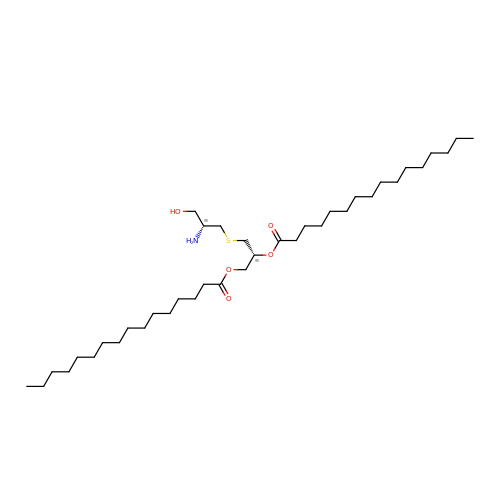(2R)-3-{[(2R)-2-AMINO-3-HYDROXYPROPYL]THIO}PROPANE-1,2-DIYL DIHEXADECANOATE | C38 H75 N O5 S | BRVXVNDGAKVNMP-LQFQNGICSA-N> MGKNTSFVLDEHYSAFIDGEIAAGRYRSASEVIRSALRLLEDRETQLRALREALEAGERSG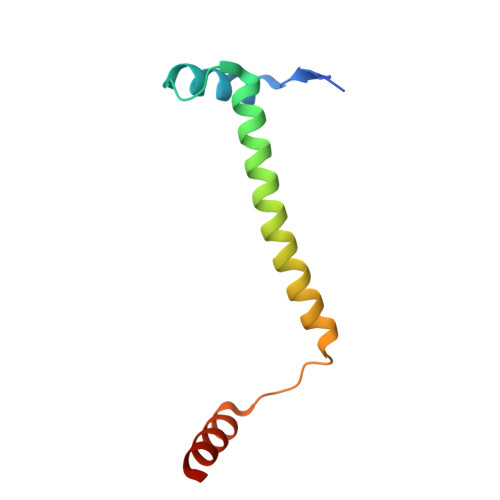SSTPFDFDGFLGRKRADASRGR(2R)-2-azanyl-3-[(2R)-2-azanyl-3-oxidanyl-3-oxidanylidene-propyl]sulfanyl-propanoic 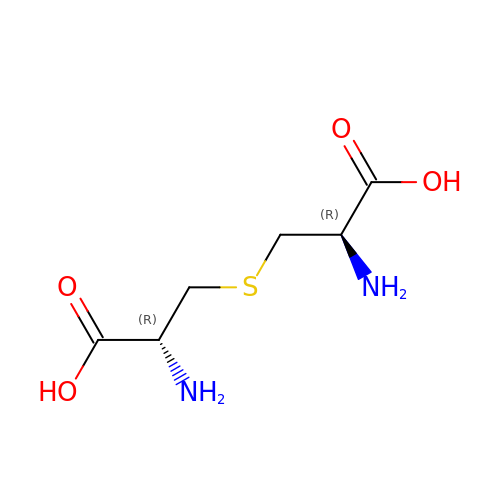acid | C6 H12 N2 O4 S | DWPCPZJAHOETAG-IMJSIDKUSA-N U2AF2 is a critical pre-mRNA splicing factor for the early stage of spliceosome assembly at the major class of 3′ splice sites. Two central RNA recognition motifs (RRM1 and RRM2) recognize a polypyrimidine consensus sequence (Py tract) composed primarily of uridines and at lower frequencies, cytidines. Structures of the U2AF2 RNA binding domain show an “open”, side-by-side conformation of the RRMs binds to uridine-rich Py tracts. Considering that the NDD-affected residues are located near the RNA interface of U2AF2 structures, here we investigated the hypothesis that disrupted U2AF2–RNA interactions could contribute to altered pre-mRNA splicing by the recurrent NDD-associated variants. De novo mutations affecting the pre-mRNA splicing factor U2AF2 are associated with developmental delays and intellectual disabilities, yet the molecular basis is unknown. To address this question, we determined the X-ray crystal structures of Arg149Trp- and Arg150His-substituted U2AF212L bound to Py tract oligonucleotides at 1.4 Å resolutions.

The Arg149Trp, Arg150His, and Arg150Cys substitutions decreased the apparent binding affinity of U2AF212L for this consensus site by approximately three-, four-, and five-fold. The sequence of the cocrystallized Py tract (5′-phosphoryl-UU(dU)U(5Br-dU)CC-3′) corresponds to a 3′ splice site of the AdML transcript, a well-characterized substrate for in vitro pre-mRNA splicing (e.g.,9,16). Like Arg149Trp, the Arg150His substitution indirectly disrupted Arg146–RNA interactions. For the Arg150His variant, the N-terminal U2AF212L α-helix shifted closer to the oligonucleotide. Arg146 appeared to be disordered by loss of a Glu201 anchor, as shown by comparing electron density maps in. Instead, Glu201 has shifted to interact with the mutant His150. Water-mediated interactions with the mutant His150 replace direct hydrogen bonds between the WT Arg150 and the N3/O2 atoms of the penultimate nucleobase. Neither of the amino acid substitutions significantly perturbed the other site–i.e., Arg149Trp has little effect on Arg150, and Arg150His had little effect on Arg149. Instead, the NDD-associated substitutions converged on disrupting Arg146 interactions with the terminal nucleotide of the cocrystallized Py tract. Unlike WT, the Arg149Trp, Arg150Cys, or Arg150His U2AF2 variants are unable to detectably promote splicing of a minigene transcript in HEK293T cells.

> GPLGSQMTRQARHLYVGNIPFGITEEAMMDFFNAQMRLGGLTQAPGNPVLAVQINQDKNFAFLEFRSVDETTQAMAFDGIIFQGQSLKIRRPHDYQPLPGMSENPSVYVPGVVSTVVPDSAHKLFIGGLPNYLNDDQVKELLTSFGPLKAFNLVKDSATGLSKGYAFCEYVDINVTDQAIAGLNGMQLGDKKLLVQRASVGAKN MINDY1 and MINDY2 are members of the MINDY family of deubiquitinases (DUBs) that have exquisite specificity for cleaving K48-polyUb, yet we have a poor understanding of their catalytic mechanism. Here, we analyze the crystal structures of MINDY1 and MINDY2 alone and in complex with monoUb, di-, and penta-K48-polyUb, identifying 5 distinct Ub binding sites in the catalytic domain that explain how these DUBs sense both Ub chain length and linkage type to cleave K48-polyUb chains. The activity of MINDY1/2 is inhibited by the Cys-loop, and we find that substrate interaction relieves autoinhibition to activate these DUBs. We also find that MINDY1/2 use a non-canonical catalytic triad composed of Cys-His-Thr.

P138 sits in a hydrophobic pocket formed by A141, I142, L204, L208, F229, and F320 to function as an anchor point for the Cys loop. Based on these observations, we predict that P138 modulates the dynamics of the Cys loop, as it provides rigidity to the loop by anchoring itself into the hydrophobic pocket. Hence, the mutation of P138 to alanine should dislodge the hydrophobic pocket interactions and result in a more dynamic, flexible loop. To test this possibility, we determined the crystal structures of the MINDY1 P138A mutant on its own and in complex with K48-Ub2. As hypothesized, the absence of P138 results in a less-extensive engagement with the hydrophobic pocket, resulting in a more mobile Cys loop, as suggested by higher b-factors of its residues. In contrast to the WT enzyme, the P138A mutant was readily modified by UbPrg, thereby supporting our notion that the P138A mutation makes the Cys loop more flexible to reduce the steric hinderance to Ub binding. Next, we determined enzyme kinetics using fluorescently labeled K48-linked pentaUb, which revealed that MINDY1 P138A mutant is a much more active enzyme with >10-fold higher kcat and ∼3-fold lower Km compared to MINDY1 WT. A chain cleavage assay with these mutants shows that disrupted anchoring (P138A or P138G) increases chain cleavage, whereas increased hydrophobicity of the side chain impairs DUB activity.

> GPLGSPEFPGRLEMEPDFYCVKWIPWKGEQTPIITQSTNGPCALLAIMNILFLQWKVKLPPQKEVITSDELMAHLGNCLLSIKPQEKSEGLQLNFQQNVDDAMTVLPKLATGLDVNVRFTGVSDFEYTPECSVFDLLGIPLYHGWLVDPQSPEAVRAVGKLSYNQLVERIITCKHSSDTNLVTEGLIAEQFLETTAAQLTYHGLCELTAAAKEGELSVFFRNNHFSTMTKHKSHLYLLVTDQGFLQEEQVVWESLHNVDGDSCFCDSDFHLSHSLGKGPGAEGGSGSPE>MQWSGARALEALLTVAGELRGPPLQLDTGQLLKIAKRGGVTAVEAVHAWRNALTGAPLNLTPEQVVAIASHDGGKQALETVQRLLPVLCQAHGLTPQQVVAIASHDGGKQALETVQRLLPVLCQAHGLTPEQVVAIASHDGGKQALETVQALLPVLCQAHGLTPEQVVAIASNGGGKQALETVQRLLPVLCQAHGLTPQQVVAIASNGGGKQALETVQRLLPVLCQAHGLTPQQVVAIASNGGGKQALETVQRLLPVLCQAHGLTPQQVVAIASNQGGKQALETVQRLLPVLCQAHGLTPQQVVAIASNGGGKQALETVQRLLPVLCQAHGLTPQQVVAIASHDGGKQALETVQRLLPVLCQAHGLTPEQVVAIASNGGGKQALETVQRLLPVLCQAHGLTPEQVVAIASHDGGKQALETVQRLLPVLCQAHGLTPQQVVAIASNGGGRPALESIVAQLSRPDPALAALTNDHLVALACLGGRPALDAVKKLEHHHHHH[2x]

Transcription activator-like (TAL) effectors specifically bind to double stranded (ds) DNA through a central domain of tandem repeats. Each TAL effector (TALE) repeat comprises 33–35 amino acids and recognizes one specific DNA base through a highly variable residue at a fixed position in the repeat. The crystal structures of TAL effector (TALE) proteins bound to their respective target DNAs have revealed that the residue at position 13 is the only one directly involved in DNA base recognition, whereas the 12th residue stabilizes the proper loop conformation. dHax3, an engineered TALE protein, proved to be a useful scaffold for structural characterizations. We then present fifteen crystal structures of engineered dHax3 variants in complex with target DNA molecules, which elucidate the structural basis for the recognition of bases adenine (A) and guanine (G) by reported or uncharacterized TALE codes.

In addition, given the resemblance between Asn and Gln, we generated one more dHax3 variant where the base recognition residue of repeat 7 was replaced by Gln. We then attempted to co-crystallize these proteins with a modified dHax3 box element whose 7th base is changed from A to G. Four complex structures were determined at high resolutions. Gln34, just as Asn34, is able to form an H-bond to the O6 atom of G, indicating a favorable interaction. There was no report of G-recognition by Gln34. Nevertheless, an independent study showed that Gln34 is highly specific for base G, but not for base A. Therefore, Gln34 may be a good code that can discriminate G from A. It was shown that His34 is a strong code for base G, but not for base A. The structures shown here provide the molecular basis for the distinctive recognition of G and A by His34. Notably, the newly determined structures reported in this manuscript show that His34 forms H-bond with base G, but not with base A, which consolidates the genetic observation that His34 is a strong and specific code for base G. The structures also suggest that Gln34 and Asn34 are both strong codes for base G. Gln34, highly specific for base G, was not reported before and should be further exploited. His34/Gln34 → G and Asp34 → C can be used as strong codes.> HMPSFDFDIPRRSPQEIAKGMVAIPGGTFRMGGEDPDAFPEDGEGPVRTVRLSPFLIDRYAVSNRQFAAFVKATGYVTDAERYGWSFVFHAHVAPGTPVMDAVVPEAPWWVAVPGAYWKAPEGPGSSITDRPNHPVVHVSWNDAVAYATWAGKRLPTEAEWEMAARGGLDQARYPWGNELTPRGRHRCNIWQGTFPVHDTGEDGYTGTAPVNAFAPNGYGLYNVAGNVWEWCADWWSADWHATESPATRIDPRGPETGT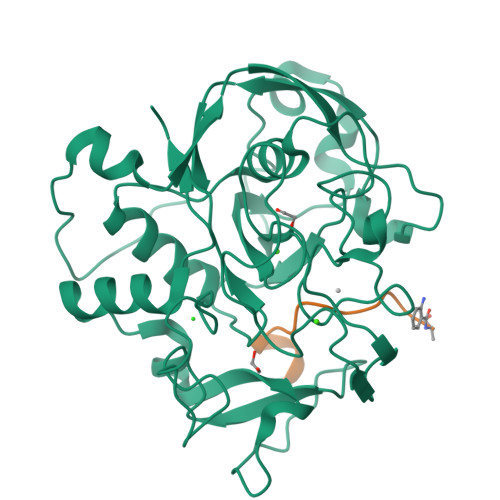ARVTKGGSFLCHESYCNRYRVAARTCNTPDSSAAHTGFRCAADP;> ATTPLCGPSRASILSG(2~{S})-4-acetamido-2-azanyl-butanoic 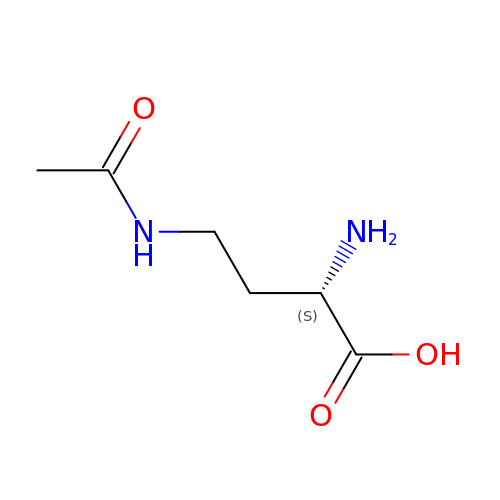acid | C6 H12 N2 O3 | YLZRFVZUZIJABA-YFKPBYRVSA-N(2-hydroxyethyl)phosphonic 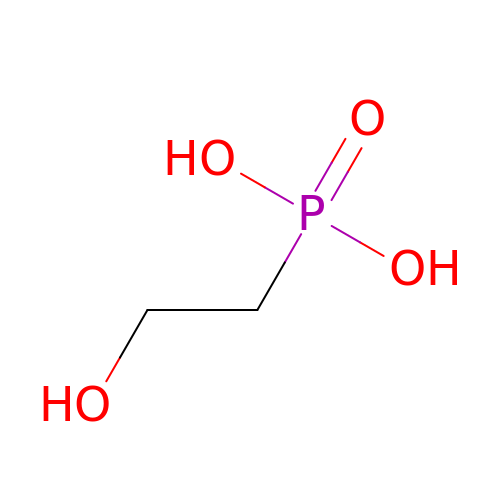acid | C2 H7 O4 P | SEHJHHHUIGULEI-UHFFFAOYSA-N>[2x]EVSTTQNDTLKVMTHNVYMLSTNLYPNWGQTERADLIGAADYIKNQDVVILNEVFDNSASDRLLGNLKKEYPNQTAVLGRSSGSEWDKTLGN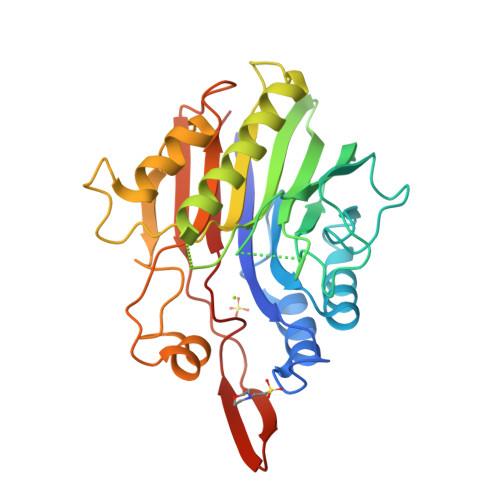YSSSTPEDGGVAIVSKWPIAEKIQYVFAKGCGPDNLSNKGFVYTKIKKNDRFVHVIGTHLQAEDSMCGKTSPASVRTNQLKEIQDFIKNKNIPNNEYVLIGGDMNVNKINAENNNDSEYASMFKTLNASVPSYTGHTATWDATTNSIAKYNFPDSPAEYLDYIIASKDHANPSYIENKVLQPKSPQWTVTSWFQKYTYNDYSDHYPVEATISMK>[2x]TIQPGTGYNNGYFYSYWNDGHGGVTYTNGPGGQF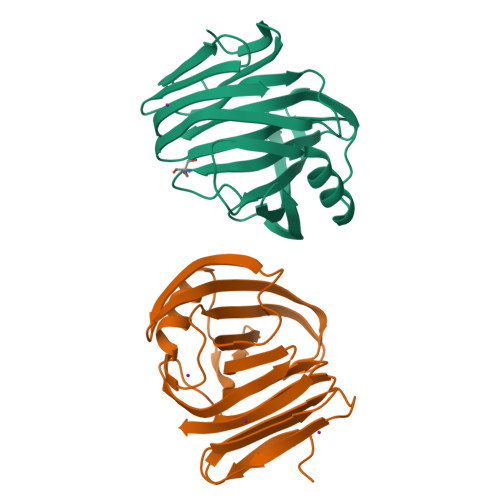SVNWSNSGNFVGGKGWQPGTKNKVINFSGSYNPNGNSYLSVYGWSRNPLIEYYIVENFGTYNPSTGATKLGEVTSDGSVYDIYRTQRVNQPSIIGTATFYQYWSVRRNHRSSGSVNTANHFNAWAQQGLTLGTMDYQIVAVEGYFSSGSASITVS> MSGQQHSSDNKNWAEKGIVIREVEILGKRPMKDIGVQQTRFDSLVLKENIALSMADILTFNSSIFVKSYGRATLSTVSFRGTSASHTQVTWNGMRINNPMLGMTDFSMIPSYFIDDASLLHGTSSVNMAGGGLGGLVKLSTVPAHQEGFGMQYVQGIGSFSTFDEFLQLKYGDKHWQISTRAVYQSSPNDYKYRNHDKKENIYDDKYNIIEQYYPIERNRSGAYKDLHILQEVYYNTGKGDRFGLNAWYTDSNRELALLTTDQGDLMDFENRQREHTLRSVLSWDHTRENWKVSARGGYVHTWLAYDYKRDLGNGIMATMTRSRSKVNTFYGQLDGEYFFSDKLLLTAGVSAHQHLVNSLDKDLNKDDNKNDKYGQGRKNDSIVYFDKGRIELSGNVSLKWQPVNRLGMSLVLRGEMFGTKWAPVIPAFFVDYVLSKRGNIMAKASITRNYRFPTLNDLYFLPGGNPALNNESGFTYETGLSFSVDKDNVYTLSGSASWFDQHINDWIIWLPTSKGFYSPVNLKKVHAYGVEVQADYAVAIDKAWKLGLNGTFAWTPSINEGEPTSKADQSVGKQLPYIPEYSATLSGRLTYRSWGLLYKWCYYSERYTMTSNAVSYTGHLPPYLMSNVTLEKGFSLRWADLSLKGTVNNLFDEEYLSVLSRPMPGINFEFFIGITPKWGKKKKGGGHHHHHH;> MKRILLSVLFIVFCLTAFVGCMKWDYGKMEPFRATGDGLFIMNEGNFQYGNATLSYYDPETKKVENEIFYRANAMKLGDVAQSMIVRDTIGWVVVNNSHVIFAISTNTFKEVGRITGLTSPRYIHFISDEKAYITQIWDYRIFIVNPKTYQITGYIECPDMTMETGSTEQMVQYGKYVYVNCWSYQNRIL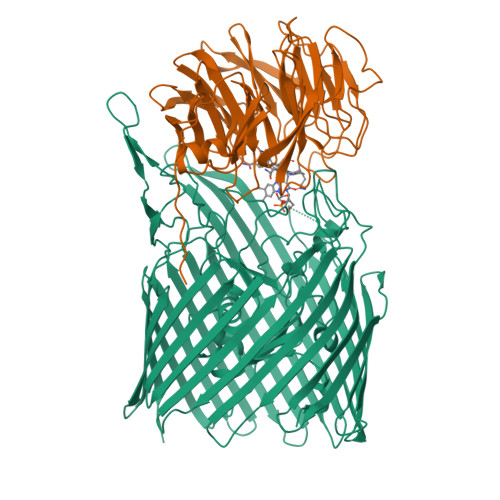KIDTTTDKVVDQLTVGIQPTSLVMDKNFKMWTITDGGYKGSPYGYEEPSLYRIDAETFKIEKQFKFQLGDAPSEVQLNGAGDELYWINKDIWRMSVDEERVPVRPFLKYRDTKYYGLTVSPKNGDVYVADAIDYQQQGMIYRYTEDGELVDEFYVGIIPGAFCWK>MELYLDTSDVVAVKALSRIFPLAGVTTNPSIIAAGKKPLDVVLPQLHEAMGGQGRLFAQVMATTAEGMVNDALKLRSIIADIVVKVPVTAEGLAAIKMLKAEGIPTLGTAVYGAAQGLLSALAGAEYVAPYVNVIDAQGGSGIQTVTDLHQLLKMHAPQAKVLAAGFKTPRQALDCLLAGCESITLPLDVAQQMISYPAVDAAVAKFEQDWQGAFGRTSITSHHHH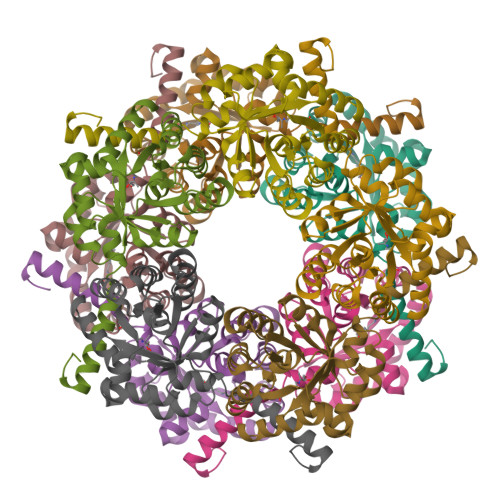H[15x]N-(2-methoxyethyl)-4-[(6-pyridin-4-ylquinazolin-2-yl)amino]benzamide | C23 H21 N5 O2 | 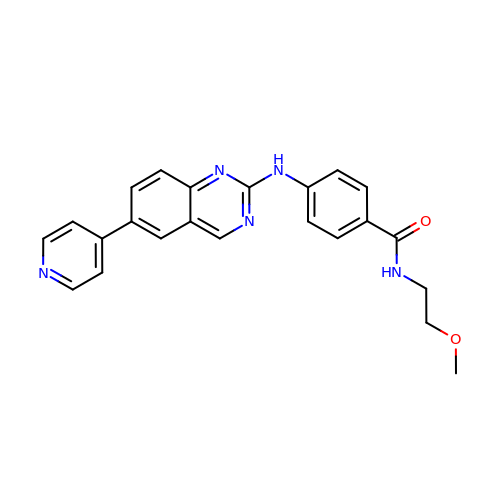NXVFABZXYFFUBF-UHFFFAOYSA-N2-acetamido-2-deoxy-alpha-D-galactopyranose | C8 H15 N 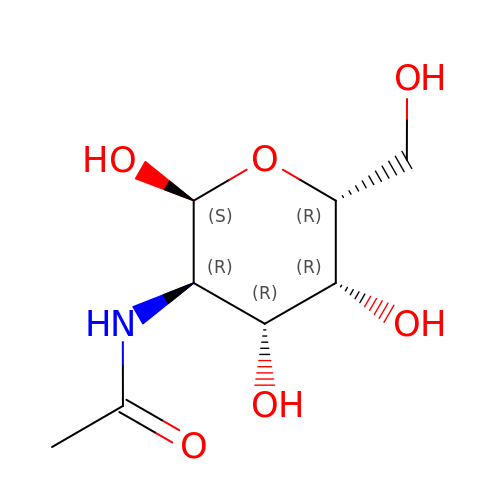O6 | OVRNDRQMDRJTHS-CBQIKETKSA-N> LEEAPWPPPEGAFVGFVLSRKEPMWADLLALAAARGGRVHRAPEPYKALRDLKEARGLLAKDLSVLALREGLGLPPGDDPMLLAYLLDPSNTTPEGVARRYGGEWTEEAGERAALSERLFANLWGRLEGEERLLWLYREVERPLSAVLAHMEATGVRLDVAYLRALSLEVAEEIARLEAEVFRLAGHPFNLNSRDQLERVLFDELGLPAIGKTEKTGKRSTSAAVLEALREAHPIVEKILQYRELTKLKSTYIDPLPDLIHPRTGRLHTRFNQTATATGRLSSSDPN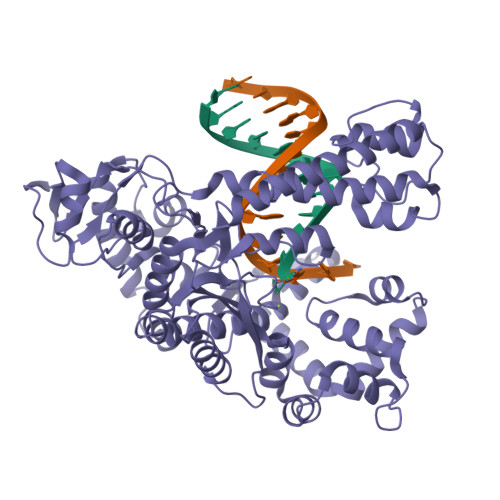LQNIPVRTPLGQRIRRAFIAEEGWLLVALDYSQIELRVLAHLSGDENLIRVFQEGRDIHTETASWMFGVPREAVDPLMRRAAKTINFGVLYGMSAHRLSQELAIPYEEAQAFIERYFQSFPKVRAWLEKTLEEGRRRGYVETLFGRRRYVPDLEARVKSVREAAERMAFNMPVQGTAADLMKLAMVKLFPRLEEMGARMLLQVHDELVLEAPKERAEAVARLAKEVMEGVYPLAVPLEVEVGIGEDWLSAKE N-acetyl-beta-muramic acid | C11 H19 N O8 | 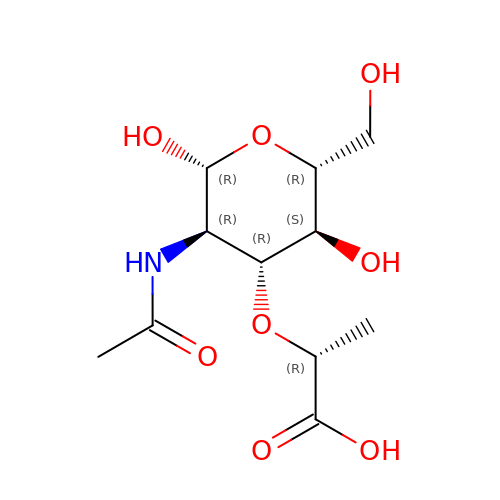MNLRQHMNZILYPY-YVNCZSHWSA-N>[8x]HMTKLADVYQ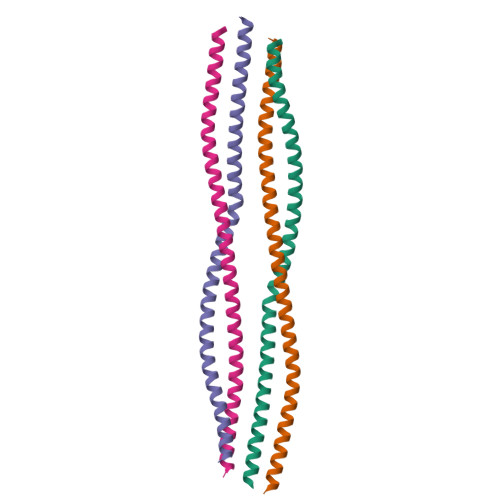AELRELRLRLDQLTANSARLEVERDNLAQDLATVRQKLQDETNLRLEAENNLAAYRQEADEATLARLDLERKIESLEEEIRFLRKIHEEEVRELQE>MKNTELEQLINEKLNSAAISDYAPNGLQVEGKETVQKIVTGVTASQALLDEAVRLGADAVIVHHGYFWKGESPVIRGMKRNRLKTLLANDINLYGWHLPLDAHPELGNNAQLAALLGITVMGEIEPLVPWGELTMPVPGLELASWIEARLGRKPLWCGDTGPEVVQRVAWCTGGGQSFIDSAARFGVDAFITGEVSEQTIHSAREQGLHFYAA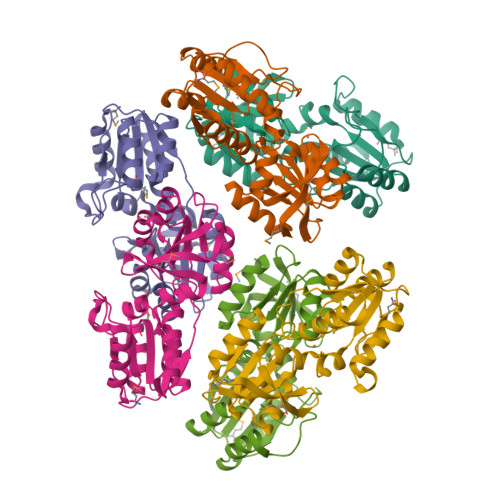GHHATERGGIRALSEWLNENTDLDVTFIDIPNPA[6x]>[4x]MSVVISDAWRQRFGGTARLYGEKALQLFADAHICVVGIGGVGSWAAEALARTGIGAITLIDMDDVCVTNTNRQIHALRDNVGLAKAEVMAERIRQINPECRVTVVDDFVTPDNVAQYMSVGYSYVIDAIDSVRPKAALIAYCRRNKIPLVTTGGAGGQIDPTQIQVTDLAKTIQDPLAAKLRERLKSDFGVVKNSKGKLGVDCVFSTEALVYPQSDGTVCAMKATAEGPKRMDCASGFGAATMVTATFGFVAVSHALKKMMAKAARQG

The enzyme responsible for t6A cyclization in E. coli was identified by comparative genomic approaches and analysis of LC/MS data sets of genomic deletion strains (ribonucleotide analysis) as CsdL, subsequently renamed to TcdA, for tRNA threonylcarbamoyladenosine dehydratase A. TcdA is an ubiquitin-activating E1-like protein with detectable homology to the adenylyltransferases MoeB and ThiF. To further the understanding of ct6A biology we have determined the high-resolution crystal structures of CsdL/TcdA in complex with AMP and ATP, an E1-like activating enzyme from Escherichia coli, which catalyzes the ATP-dependent dehydration of t6A to form ct6A. CsdL/TcdA is a dimer whose structural integrity and dimer interface depend critically on strongly bound K+ and Na+ cations. The tertiary structure of monomeric TcdA consists of seven β-strands in a continuous sheet surrounded by eight α-helices.

To shed light onto the structural basis for the tRNA binding and ct6A synthetic properties of TcdA-ATP, we determined the crystal structure of E. coli TcdA loaded with ATP to 1.77 Å resolution (R/Rfree values of 0.139/0.176) and AMP to 1.89 Å resolution (R/Rfree values of 0.141/0.183). The structure of TcdA-AMP was solved by MR using the fully refined model of the TcdA-ATP complex. Besides localized changes in the active site, the TcdA-ATP and TcdA-AMP structures are identical (RMSD 0.16 Å over 246 Cα atoms). In the TcdA-AMP complex, the nucleotide-binding residues stabilize AMP in a manner analogous to ATP, with no conformational changes in the TcdA dimer. In the TcdA-ATP and TcdA-AMP complexes, the region between β7 and the C-terminal α8 spanning residues 214–236 is fully disordered in electron density maps. The first 310 helix (H310a) contains three residues that are conserved in the MoeB/E1 superfamily, including a strictly conserved Asn69 that interacts with bound ATP/AMP via water-mediated hydrogen bonds. In particular, the P loop and the residues that contact ATP/AMP are nearly strictly conserved across all structural homologs. A second metal binding site specific for Na+ is found at the dimer interface in an octahedral coordination. The Na+ cation is axially liganded by the carbonyl oxygens of two symmetric Thr162 residues that lie in a short 310 helix segment (H310c) from opposite monomers, with four water molecules occupying the equatorial positions.> GPGSGQLLFANFNQDNTSLAVGSKSGYKFFSLSSVDKLEQIYECTDTEDVCIVERLFSSSLVAIVSLKAPRKLKVCHFKKGTEICNYSY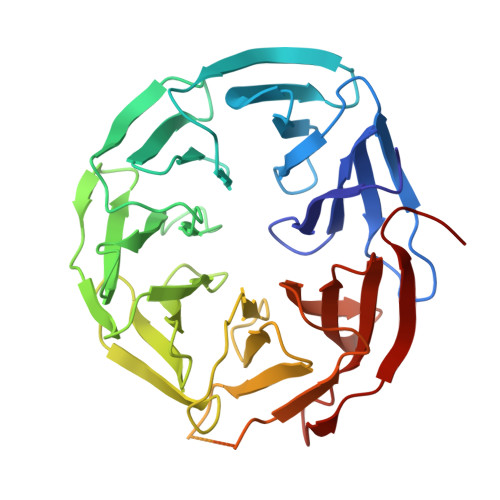SNTILAVKLNRQRLIVCLEESLYIHNIRDMKVLHTIRETPPNPAGLCALSINNDNCYLAYPGSATIGEVQVFDTINLRAANMIPAHDSPLAALAFDASGTKLATASEKGTVIRVFSIPEGQKLFEFRRGVKRCVSICSLAFSMDGMFLSASSNTETVHIFKLETVKEKPPEEPTTWTGYFGKVLMASTSYLPSQVTEMFNQGRAFATVRLPFCGHKNICSLATIQKIPRLLVGAADGYLYMYNLDPQEGGECALMKQHRLDGSLV>LKARGGPKTLRRTPGVEPKDIRVLPGPLGSGNFGTVFRGVFKGDQDVVLKNAKADVMAAEELLECEMDVNYHVHANAKGTCARFMGCIELGAKDGGEIYNGTLTEGLWLMWANEGENTVEALMRRGTAPLATAMACADATELGVTKKAMRELLGSLARLHECGVVHRDVKPANLIAAEKDGGVLKLIDLGAAALCLPLPETLNYYPGDGPADPRYAKADELYL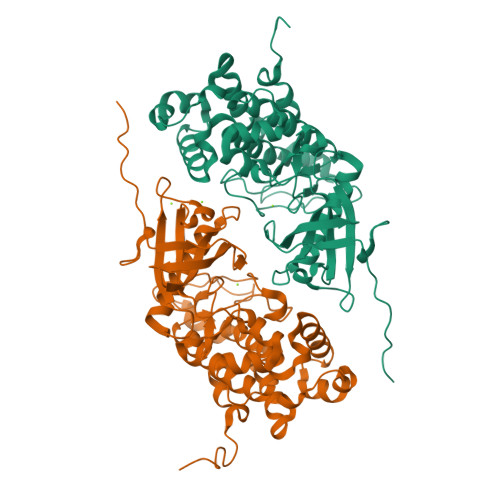LPPGSPRPTKDNAAKLWEAHKPDRFDSWSAGCVMLQLAVVGLRTDAGLERFLADYKAVGYDVNAFRGEKSGEYGTMDFAALDANGGAGWDLCQRLMEAERDARASCEAALSHAFFDAAALEHHHHHH[2x]> MADEIDAMALYRAWQQLDNGSCAQIRRVSEPDELRDIPAF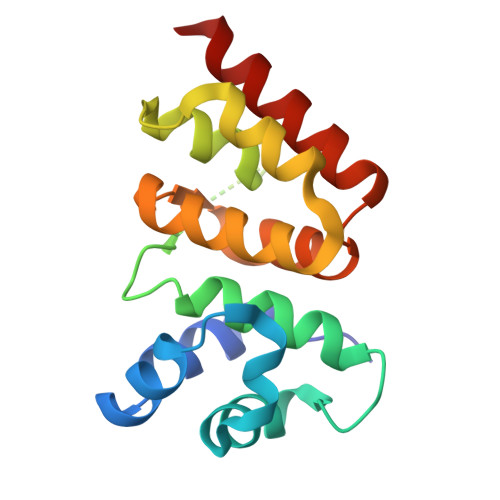YRLVQPFGWENPRHQQALLRMVFCLSAGKNVIRHQDKKSEQTTGISLGRALANSGRINERRIFQLIRADRTADMVQLRRLLTHAEPVLDWPLMARMLTWWGKRERQQLLEDFVLTTNKNA> AIET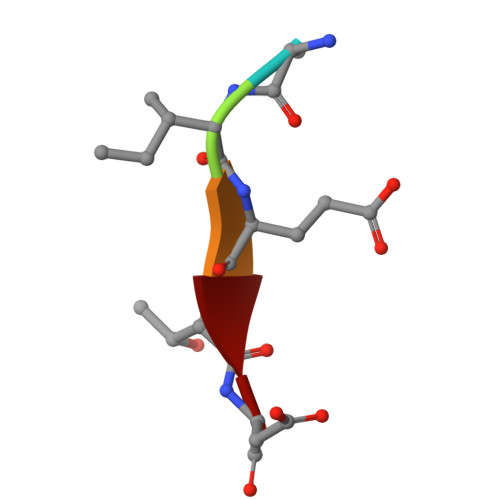D> EVPAD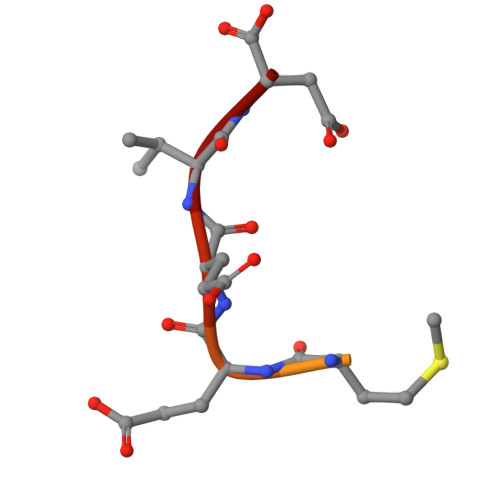TEMEEVD B12 is obtained from food and travels from the stomach, through the intestine, and into the bloodstream by three B12-transporting proteins: salivary haptocorrin (HC), gastric intrinsic factor, and transcobalamin (TC), which all bind B12 with high affinity and require proteolytic degradation to liberate Cbl. B12 uptake is a finely orchestrated process involving a number of structurally related high-affinity B12-binding proteins, which protect B12 and carry it through cell membranes via specific protein–receptor interactions. Like the previously elucidated bovine and human TC-Cbl structures, recombinantly expressed rat TC consists of two domains: (i) an N-terminal, disulfide-bonded, α-helical six-hairpin glycosidase-like α-domain and (ii) a C-terminal β-stranded ubiquitin-like β-domain, the two linked by an interdomain loop. In the shown structure, Cbl is sandwiched between the α- and β-domains of rTC in a base-on conformation.

In this paper, we present the complex crystal structure between rat transcobalamin (rTC) and GSCbl. We obtained crystals of rTC that diffracted to 1.2 Å resolution at pH 5.5 in the presence of GSH and to our surprise we observed continuous electron density emanating from the Co of the Cbl ring system corresponding to GSH. GSH binds at the β-axial site, located between Cbl and the α-domain of rTC. Therefore, most interactions are formed with residues located in the α-domain. The Co–S bond is approximately 2.4 Å, the Co–dimethylbenzimidazole base bond is 2.2 Å and the corrin fold angle is 6.6°, which is defined as the butterfly angle between N21, C4, C5, C6, N22 C9, C10, and C10, C11, N23, C14, C15, C16, and N24. The majority of the 14 polar interactions between GSH and rTC are formed through solvent molecules. However, direct side chain interactions are present between Ser195, Thr198, and GSH. The strongest interaction is found between the α-helix dipole of α6 (Tyr154 and Tyr155), which interacts with the carboxylate of the γ-glutamate group of GSH. When the β site of Cbl is occupied by a strong ligand such as cyanide or GSH, the TC α7/α8 loop is disordered (bovine TC) or folds outward into the solvent (rat and human TC) and forms little hydrogen bonds with the rest of the protein. Our structure of rTC in complex with GSCbl clearly displays the broad specificity of TC concerning β groups of Cbl.

> GSSHHHHHHSSGDDDDKGEFCVIPKMDGQLVEKLGQRLLPWMDRLSSEQLNPSIYVGLRLSSMQAGTKENLYLHNLKLHYQQCLLRSTSSDDNSGCQTKISGGSLALYLLALRANCELLGSRKGDRMVSQLKWFLEDEKKAIGHHHEGHPHTSYYQYGLSILALCVHRKRVHDSVVGKLLYAVEHDYFTYQGHLSVDTEAMAGLAFTCLERFNFNSDLRPRITTAIETVREKILKAQAPEGYFGNIYSTPLALQMLMTSPGVGLGPACLKARKSLLLSLQDGAFQNPMMISQLLPVLNHKTYLNLISPDCQAPRVMLVPATEDPVHLSEVSVTLKVSSVLPPYERTVSVFAGASLEDVLNRARDLGEFTYGTQASLSGPYLTSVLGKEAGDREYWQLLRVPDTPLLQGIADYKPKNGETIELRLVKM>MHHHHHHSSGLVPRGSEDKWRNAFDHMLMEEFEEKMDQIEHGLLMLSE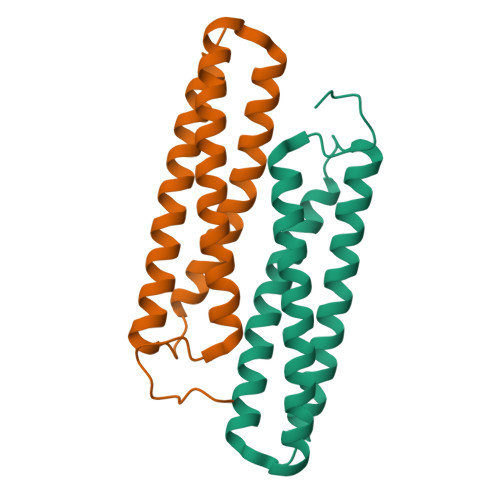QYKELEKTKSKELKEQILRELTIAENYLRGALKFMQQEAKRTDLNMFERYNFETAVSTIEILVKDLAELAKKVKAVKSDD[4x]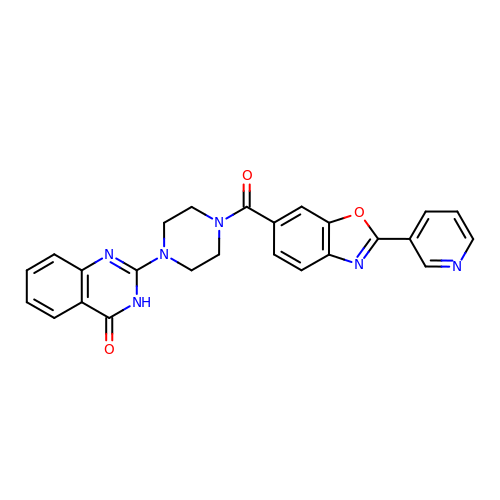2-[4-[(2-pyridin-3-yl-1,3-benzoxazol-6-yl)carbonyl]piperazin-1-yl]-3~{H}-quinazolin-4-one | C25 H20 N6 O3 | NEEKCMPINYYRAZ-UHFFFAOYSA-N4-methoxy-3-[2-[(3-methoxy-4-morpholin-4-yl-phenyl)amino]pyridin-4-yl]benzenecarbonitrile 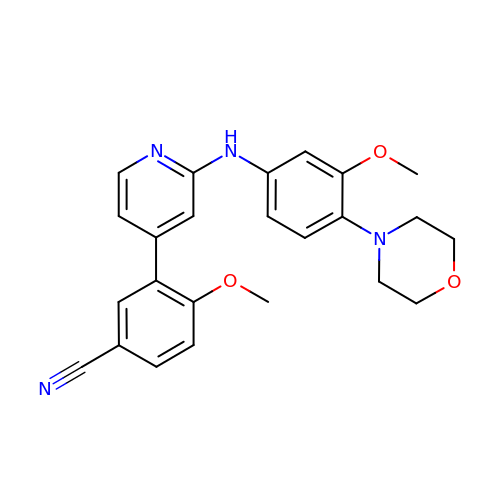| C24 H24 N4 O3 | JKDVQSBZXOTCNO-UHFFFAOYSA-N> MTDLSSLIETADLRLLLTTVPTETEALY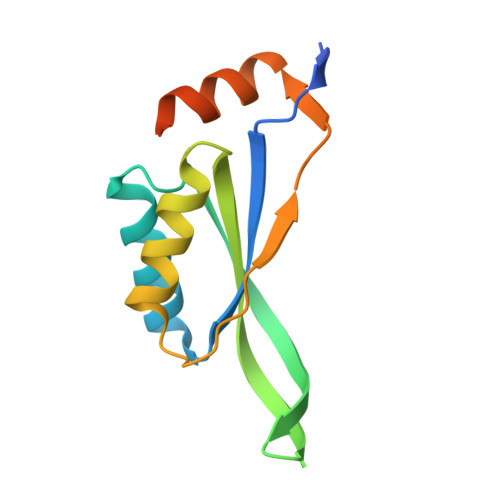LALAAVEKGLAAEVLITPVTRVRRENGKLVVEDVYRLSFKTTRERLDALVAWLQRRHPLALPECLVLTPIASSVAYRDWLRSSLQGGSHHWGGHHHHHH>[2x]MENTENSVDSKSIKNLEPKIIHGSESMDSGISLDNSYKMDYPEMGLCIIINNKNFHKSTGMTSRSGTDVDAANLRETFRNLKYEVRNKNDLTREEIVELMRDVSKEDHSKRSSFVCVLLSHGEEGIIFGTNGPVDLKKITNFFRGDRCRSLTG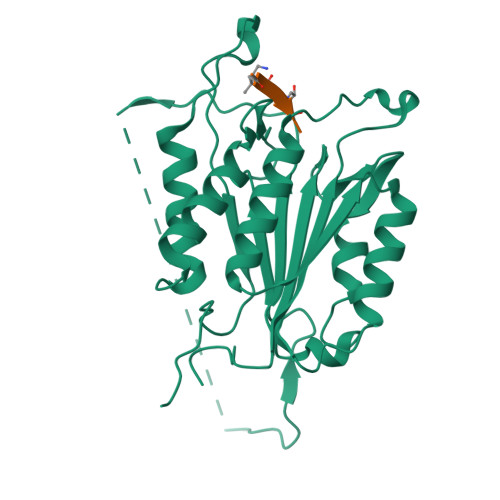KPKLFIIQACRGTELDCGIETDSGVDDDMACHKIPVEADFLYAYSTAPGYYSWRNSKDGSWFIQSLCAMLKQYADKLEFMHILTRVNRKVATEFESFSFDATFHAKKQIPCIVSMLTKELYFYHQLHHHHHH>[2x]XGEIAQQLKEIAKQLKEIAWQLKEIAQQLKGX

αHBs are oligomers of 5 or more α-helical peptides that assemble into coiled-coil structures with central solvent-accessible channels. We targeted two properties of αHBs: oligomeric state, which directly affects the internal diameter of the channel; and the identities of channel-facing residues, which fine tune this dimension and introduce different chemistries. The αHBs are loaded with an environment sensitive dye (in this case, 1,6-diphenyl-1,3,5-hexatriene, DPH) that binds within the channels and fluoresces. Accordingly, challenging the array with analytes leads to differential displacement of the dye across the array to give a fluorescent fingerprint.

Therefore, we kept e = Ala in most designs and made g = Ala, Asn, Gln, Glu, Ile or Ser to sample oligomer states of 5–8 and internal diameters of ≈5–10 Å27,34. Despite the requirements for aliphatic residues at a and d, up to 40% of these can be changed to other side chains without compromising barrel integrity. We introduced mutations at one or two of these sites to generate four groups of αHB: Group I had entirely hydrophobic interiors, but with different sizes and shapes of channel; Groups II and III had polar uncharged or polar charged residues, respectively, at specific points along the channel; and Group IV had aromatic residues installed in their channels. Finally, one third of the designs were crystallized and yielded 12 X-ray crystal structures, all of which were open αHBs with fully accessible channels.1-methyl-4-(1-methylethyl)benzene 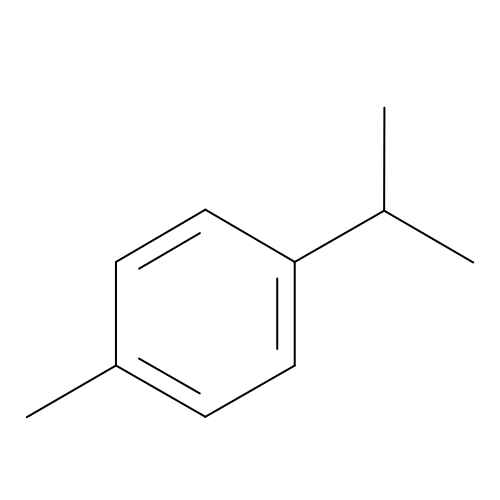| C10 H14 | HFPZCAJZSCWRBC-UHFFFAOYSA-N> MENGYTYEDYKNTAEWLLSHTKHRPQVAIICGSGLGGLTDKLTQAQIFDYSEIPNFPRSTVPGHAGRLVFGFLNGRACVMMQGRFHMYEGYPLWKVTFPVRVFHLLGVDTLVVTNAAGGLNPKFEVGDIMLIRDHINLPGFSGQNPLRGPNDERFGDRFPAMSDAYDRTMRQRALSTWKQMGEQRELQEGTYVMVAGPSFETVAECRVLQKLG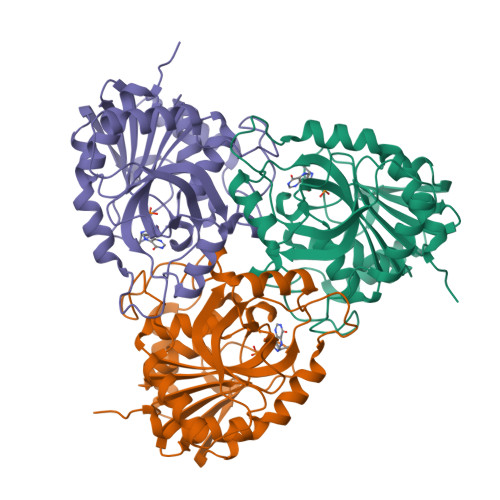ADAVGMSTVPEVIVARHCGLRVFGFSLITNKVIMDYESLEKANDEEVLAAGKQAAQKLEQFVSILMASIPLPDKAS1,3,4,9-TETRAHYDRO-2-(HYDROXYBENZOYL)-9-[(4-HYDROXYPHENYL)METHYL]-6-METHOXY-2H-PYRIDO[3,4-B]INDOLE 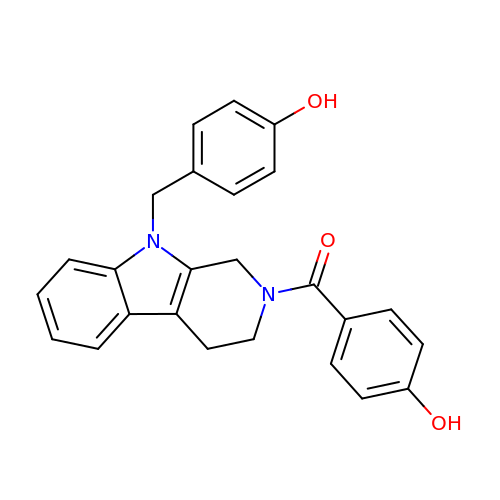| C25 H22 N2 O3 | ADXYEWMDAGIULV-UHFFFAOYSA-N>[2x]GSPEKILAQIIQEHREGLDWQEAATRASLSLEETRKLLQSMAAAGQVTLLRVENDLYAISTERYQAWWQAVTRALEEFHSRYPLRPGLAREELRSRYFSRLPARVYQALLEEWSREGRLQ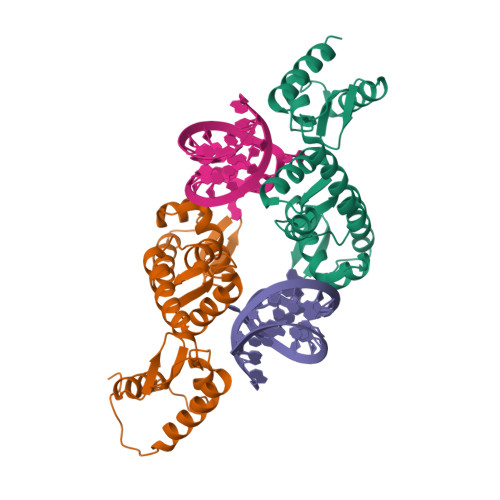LAANTVALAGFTPSFSETQKKLLKDLEDKYRVSRWQPPSFKEVAGSFNLDPSELEELLHYLVREGVLVKINDEFYWHRQALGEAREVIKNLASTGPFGLAEARDALGSSRKYVLPLLEYLDQVKFTRRVGDKRVVVGN> SNAMLGLKRFRLPALASAAFIALGAGTAAAQSNVVIMQDPGGGYGDALRKVMYDPFEKETGIKVVTVQEARSGPRIKAQAEAGK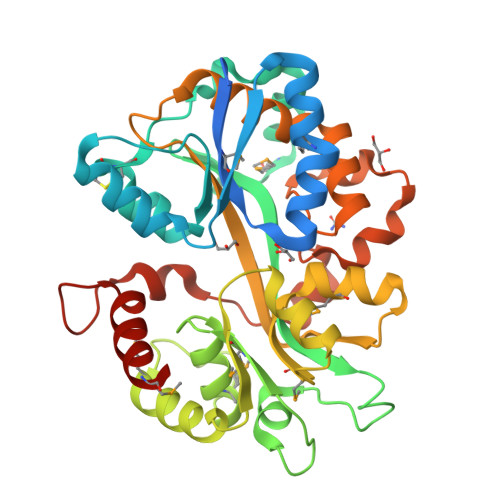AQWDLTFIFDQETKLLGDCCLADIDYSKLSESAHKTLAAMPDNLKRKKGVALQVIGVGLVYNKDKFKGDKAPQTWADFWDVKKFPGRRCMPAWPRFTFEAALMADGVTKDKLYPIDMDRALKKLKEIKPHVVKWWTTAAQPPQLILDGEADMCLAYTGSMSKLALEGAPIDLTFNQGFVYYDFFSIPKGAPNYDNALKLLSWRLDPKRAAQLTSTFPVALPSKVVFDAATDKNIARYWANNPENVAKAIEWSPDFWGAPSPAGNSTNEEYGQEKLNAMLAQ The S. solfataricus protein Sso2509 is a translation recovery factor (Trf) that interacts with aIF2 and is responsible for the release of aIF2 from bound mRNAs, thereby enabling translation re‐initiation. It is a member of the domain of unknown function 35 (DUF35) protein family and is conserved in Sulfolobales as well as in other archaea. aIF2 has a second function: It protects leaderless mRNAs against degradation by binding to their 5′‐ends.

Here, we present the X‐ray structure of S. solfataricus Trf solved to a resolution of 1.65 Å. Trf is composed of an N‐terminal rubredoxin‐like domain containing a bound zinc ion and a C‐terminal oligosaccharide/oligonucleotide binding fold domain. The Trf structure reveals putative mRNA binding sites in both domains. Surprisingly, the Trf protein is structurally but not sequentially very similar to proteins linked to acyl‐CoA utilization—for example, the Sso2064 protein from S. solfataricus—as well as to scaffold proteins found in the acetoacetyl‐CoA thiolase/high‐mobility group‐CoA synthase complex of the archaeon Methanothermococcus thermolithotrophicus and in a steroid side‐chain‐cleaving aldolase complex from the bacterium Thermomonospora curvata. This suggests that members of the DUF35 protein family are able to act as scaffolding and binding proteins in a wide variety of biological processes.

>MREEEIRELYFKYFDENKLPFIQCNKCGHKFYYPRVLCPKCGSSDIEVRFSKGLGKIFAMTKVYRKDGSYVIYGIVELEEGFRMYSNIIEESQADINRKVEVIFKEINGKKYPLFKTVT[2x]> MKKVRLKELESRLQQVDGFEKPKLLLEQYPTRPHIAACMLYTIHNTYDDIENKVVADLGCGCGVLSIGTAMLGAGLCVGFDIDEDALEIFNRNAEEFELTNIDMVQCDVCLLS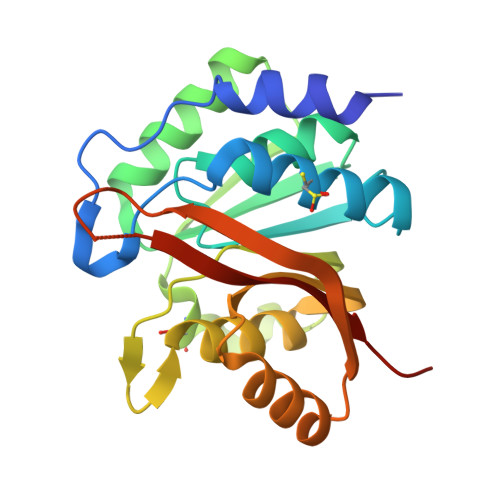NRMSKSFDTVIMNPPFGTKNNKGTDMAFLKTALEMARTAVYSLHKSSTREHVQKKAAEWKIKIDIIAELRYDLPASYKFHKKKSVDIEVDLIRFSFHHHHHH(5,6-dimethyl-1H-benzimidazol-2-yl)methanol | 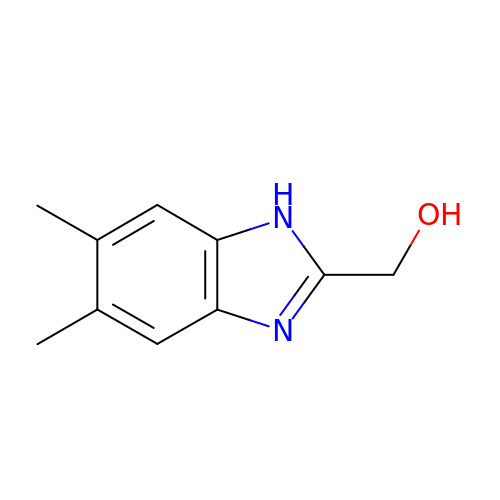C10 H12 N2 O | NLTYZPBQHXXZGL-UHFFFAOYSA-N> MAQILPIRFQEHLQLQNLGINPANIGFSTLTMESDKFICIREKVGEQAQVVIIDMNDPSNPIRRPISADSAIMNPASKVIALKAGKTLQIFNIEMKSKMKAHTMTDDVTFWKWISLNTVALVTDNAVYHWSM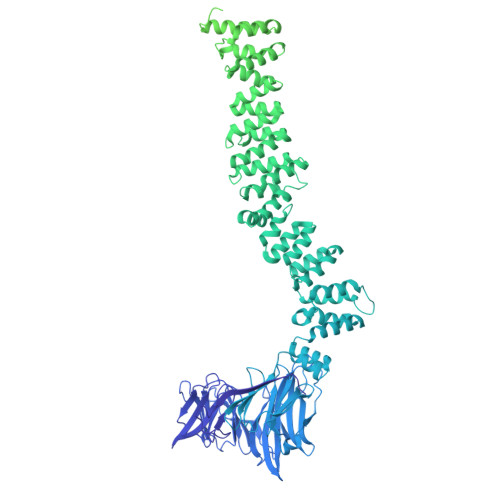EGESQPVKMFDRHSSLAGCQIINYRTDAKQKWLLLTGISAQQNRVVGAMQLYSVDRKVSQPIEGHAASFAQFKMEGNAEESTLFCFAVRGQAGGKLHIIEVGTPPTGNQPFPKKAVDVFFPPEAQNDFPVAMQISEKHDVVFLITKYGYIHLYDLETGTCIYMNRISGETIFVTAPHEATAGIIGVNRKGQVLSVCVEEENIIPYITNVLQNPDLALRMAVRNNLAGAEELFARKFNALFAQGNYSEAAKVAANAPKGILRTPDTIRRFQSVPAQPGQTSPLLQYFGILLDQGQLNKYESLELCRPVLQQGRKQLLEKWLKEDKLECSEELGDLVKSVDPTLALSVYLRANVPNKVIQCFAETGQVQKIVLYAKKVGYTPDWIFLLRNVMRISPDQGQQFAQMLVQDEEPLADITQIVDVFMEYNLIQQCTAFLLDALKNNRPSEGPLQTRLLEMNLMHAPQVADAILGNQMFTHYDRAHIAQLCEKAGLLQRALEHFTDLYDIKRAVVHTHLLNPEWLVNYFGSLSVEDSLECLRAMLSANIRQNLQICVQVASKYHEQLSTQSLIELFESFKSFEGLFYFLGSIVNFSQDPDVHFKYIQAACKTGQIKEVERICRESNCYDPERVKNFLKEAKLTDQLPLIIVCDRFDFVHDLVLYLYRNNLQKYIEIYVQKVNPSRLPVVIGGLLDVDCSEDVIKNLILVVRGQFSTDELVAEVEKRNRLKLLLPWLEARIHEGCEEPATHNALAKIYIDSNNNPERFLRENPYYDSRVVGKYCEKRDPHLACVAYERGQCDLELINVCNENSLFKSLSRYLVRRKDPELWGSVLLESNPYRRPLIDQVVQTALSETQDPEEVSVTVKAFMTADLPNELIELLEKIVLDNSVFSEHRNLQNLLILTAIKADRTRVMEYINRLDNYDAPDIANIAISNELFEEAFAIFRKFDVNTSAVQVLIEHIGNLDRAYEFAERCNEPAVWSQLAKAQLQKGMVKEAIDSYIKADDPSSYMEVVQAANTSGNWEELVKYLQMARKKARESYVETELIFALAKTNRLAELEEFINGPNNAHIQQVGDRCYDEKMYDAAKLLYNNVSNFGRLASTLVHLGEYQAAVDGARKANSTRTWKEVCFACVDGKEFRLAQMCGLHIVVHADELEELINYYQDRGYFEELITMLEAALGLERAHMGMFTELAILYSKFKPQKMREHLELFWSRVNIPKVLRAAEQAHLWAELVFLYDKYEEYDNAIITMMNHPTDAWKEGQFKDIITKVANVELYYRAIQFYLEFKPLLLNDLLMVLSPRLDHTRAVNYFSKVKQLPLVKPYLRSVQNHNNKSVNESLNNLFITEEDYQALRTSIDAYDNFDNISLAQRLEKHELIEFRRIAAYLFKGNNRWKQSVELCKKDSLYKDAMQYASESKDTELAEELLQWFLQEEKRECFGACLFTCYDLLRPDVVLETAWRHNIMDFAMPYFIQVMKEYLTKVDKLDASESLRKEEEQATETQ> HDDFADDI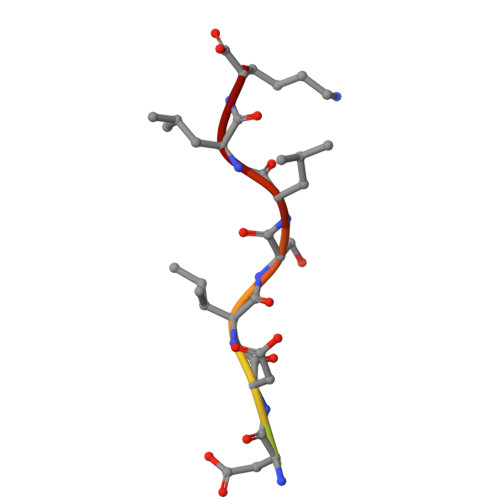SLLK> CAAGAGCCTGATCGGACAAGC;> AGCCTACCTGGCAGGACGACTCTCTGCACTACTACGTCAGCA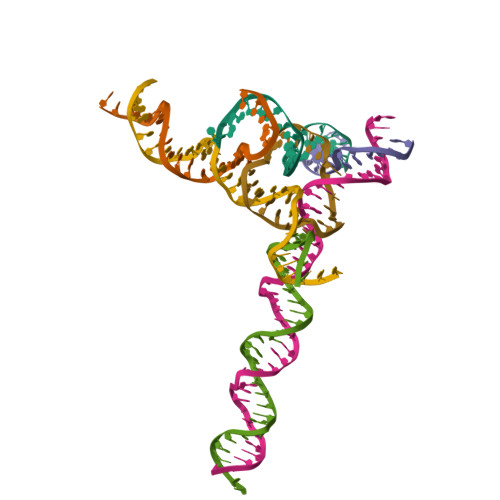;> CACGAGCCTGATCGGACATCACATGCTGAGT;> TCGCTTGTGGTAGG;> TCACTCAGCATGTGATGTGGCTCT;> TTTGCTGACGTAGTAGTGCAGAGAGTCGTGGCTCG;> GCCACCGATCACCGATCACCT> MRSGDAEIKGIKPKVIEEYSLSQGSGPSNDSWKSLMSSAKDTPLQYDHMNRESLKKYFDP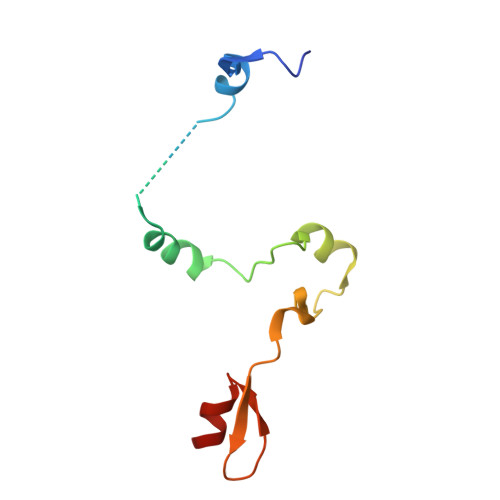NAQLIEDPLDKPIQYRVCEKCGKPLALTAIVDHLEN> CSLDNGGCDQFCREERSEVRCSCAHGYVLGDDSKSCVSTERFP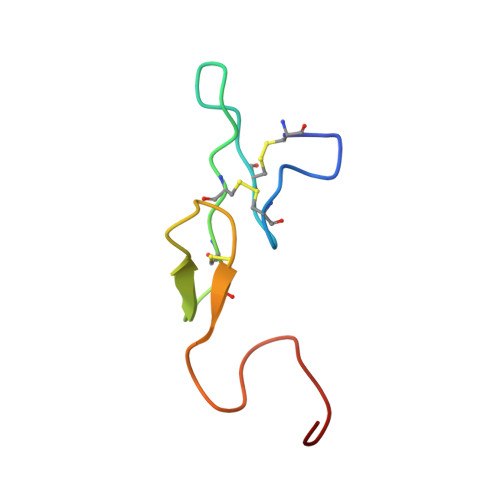CGKFTQGR>MSELSAIETAAAIAGGSMTALEACDAAIARIEQRDGPINAVVVRDFDRAREAAKAADGEVAAGVSKPLLGVPMTIKESIDIAGLPTSWGFAEHADHIATADSVVVSRLKAAGAVFLGKTNIPVALADWQSSNPNYGRTNNPHDLTRSAGGSSGGAAAALAAGMVPLEYGSDIGGSIRVPAHFCGVWGLKTTFDAVSLEGHYLPRTDGARGELGVVGPMARNPQDLALALDLTSRIALPIARIDTLNGLRILLLTHHPRAAADSAVVAAVEKAAESCAAQGAQVSTSNADLPDLSKLVSDYTRM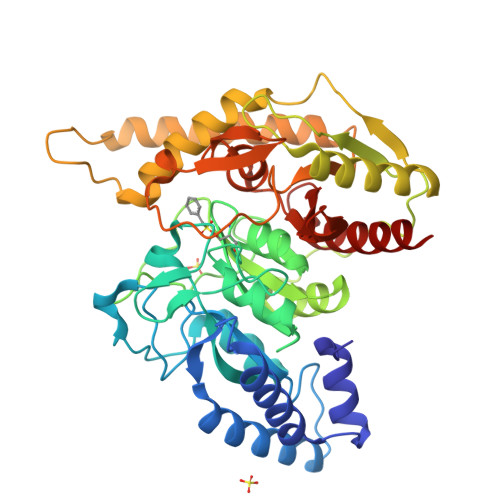LLIVLAQGKAPEGTEPVSLNAWYGMLDDQARTIRGFDRLFDSFDAIFCPVLGTSAFPHSDEADWGKRTLTIDGADTPFGSQLAWISMATYCGMPALSMPVGTDANGLPIGLQIITRNWSDHDAVRIGALVADALAA[2x]> PVITVNTNVAEKSIPVFFQAALTNMMTKALQKPKEVMFVDLRSGANIMMGGDRNPCVFATVECIGRLNPTSNLAMARDMEDMFIEHLNVRRERIVIRFIPV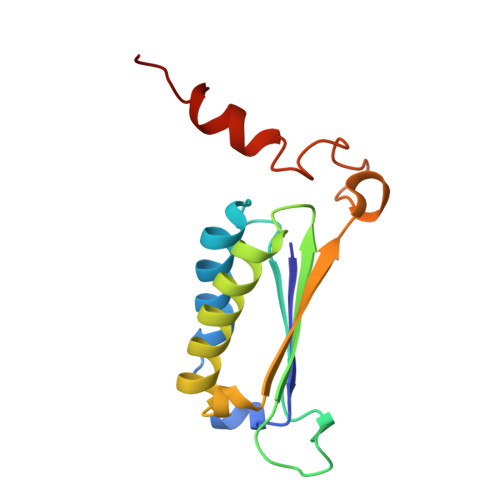PALFCSFNGALHDVSIERDEDIISQAIAEYLHA> GPLGSPLTASMLASAPPQEQKQMLGERLFPLIQAMHPTLAGKITGMLLEIDNSELLHM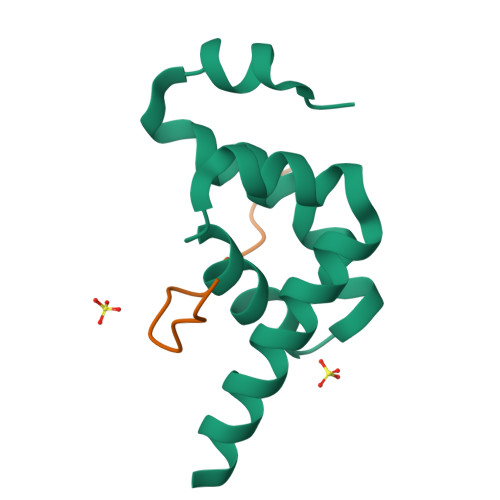LESPESLRSKVDEAVAVLQAHQAKEAAQKA;> FVPNVHAAEFVPSFL>[8x]MATQGVFTLPANTRFGVTAFANSSGTQTVNVLVNNETAATFSGQSTNNAVIGTQVLNSGSSGKVQVQVSVNGRPSDLVSAQVILTNELNFALVGSEDGTDNDYNDAVVVINWPLG;>KKLLKLLKLLLX[8x]

Herein we report the first X-ray crystal structures of mixed chirality α-helices in short peptides comprising only natural residues as the example of a stapled bicyclic and a linear membrane disruptive amphiphilic antimicrobial peptide (AMP) containing seven l- and four d-residues, as complexes of fucosylated analogs with the bacterial lectin LecB. The mixed chirality α-helices are superimposable onto the homochiral α-helices and form under similar conditions as shown by CD spectra and MD simulations but non-hemolytic and resistant to proteolysis. To get a direct insight into the structure of AMBP bp65/bp69 and their linear analogs ln65/ln69, we performed several crystallization studies using either the compounds themselves or their racemates to be crystallized as pure compounds, or their fucosylated derivatives of both mirror image peptides as complexes with the P. aeruginosa lectin LecB. While previous reports of similar mixed chirality AMPs concluded on either unordered conformations or helical conformations appearing in a membrane environment based on deconvolution of FTIR spectra, here we reported X-ray crystallographic evidence of short mixed chirality helices consisting of only natural residues existing as helix bundles within the protein environment of a lectin and almost perfectly superimposable with their parent homochiral α-helices. These direct observations unequivocally demonstrate that the α-helical fold with only natural residues can sometimes tolerate multiple stereochemical inversions without significant conformational changes.

The LecB complex with the homochiral sequence Fln65 showed eight crystallographically distinct structures, which represented amphiphilic α-helices. The same was true across the ten different X-ray structures of linear α-helices observed in the X-ray structures of LecB complexes for the homochiral Fln65 and its mixed chirality analog Fdln69 (RMSD < 0.9 Å). This comparison showed that the helical geometries of the homochiral and heterochiral helices were not significantly different from each other. In the case of bp65, bp71 and Fln65 the peptides were aggregated in bundles of four of more helices via hydrophobic contacts between leucine side chains. A closer analysis of the different X-ray structures showed that the peptides did not make any significant contact with LecB apart from the anchoring fucose residue. Indeed, bp65 showed a CD (circular dichroism) spectrum typical for an α-helical AMP, with a transition from an unordered conformation in water to an α-helical conformation upon addition of up to 20% v/v trifluoroethanol (TFE) or in the presence of 5 mM n-dodecylphosphocholine (DPC) micelles mimicking the membrane environment.> MSAALPSIQLPVDYNNLFNEITDFLVTFKQDTLSSDATRNENEDENLDAENIEQHLLEKGPKYMAMLQKVANRELNSVIIDLDDILQYQNEKFLQGTQADDLVSAIQQNANHFTELFCRAIDNNMPLPTKEIDYKDDVLDVILNQRRLRNERMLSDRTNEIRSENLMDTTMDPPSSMNDALREVVEDETELFPPNLTRRYFLYFKPLSQNCARRYRKKAISSKPLSVRQIKGDFLGQLITVRGIITRVSDVKPAVEVIAYTCDQCGYEVFQEVNSRTFTPLSECTSEECSQNQTKGQLFMSTRASKFSAFQECKIQELSQQVPVGHIPRSLNIHVNGTLVRSLSPGDIVDVTGIFLPAPYTGFKALKAGLLTETYLEAQFVRQHKKKFASFSLTSDVEERVMELITSGDVYNRLAKSIAPEIYGNLDVKKALLLLLVGGVDKRVGDGMKIRGDINVCLMGDPGVAKSQ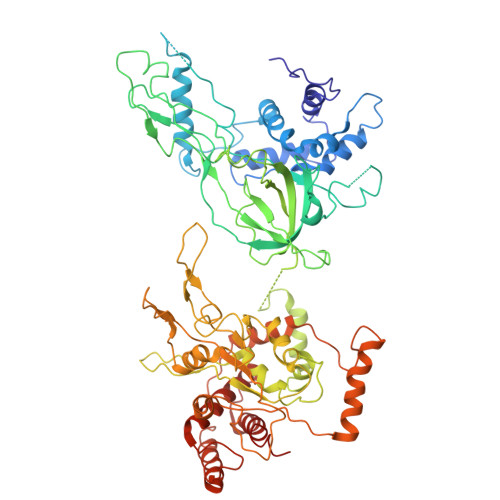LLKAICKISPRGVYTTGKGSSGVGLTAAVMKDPVTDEMILEGGALVLADNGICCIDEFDKMDESDRTAIHEVMEQQTISISKAGINTTLNARTSILAAANPLYGRYNPRLSPLDNINLPAALLSRFDILFLMLDIPSRDDDEKLAEHVTYVHMHNKQPDLDFTPVEPSKMREYIAYAKTKRPVMSEAVNDYVVQAYIRLRQDSKREMDSKFSFGQATPRTLLGIIRLSQALAKLRLADMVDIDDVEEALRLVRVSKESLYQ N-[(3S)-2-oxotetrahydrofuran-3-yl]decanamide 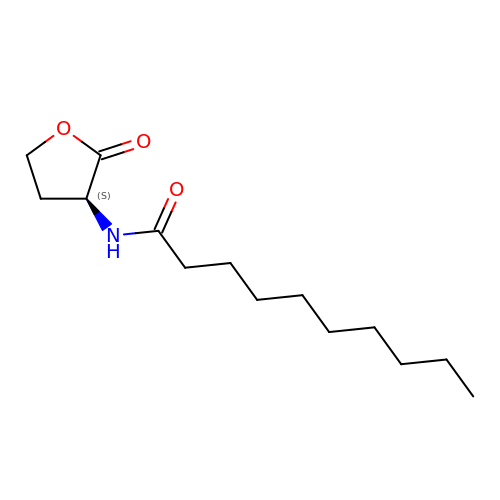| C14 H25 N O3 | TZWZKDULKILUPV-LBPRGKRZSA-N PHOSPHORIC ACID MONO-[2-AMINO-3-(3H-IMIDAZOL-4-YL)-PROPYL]ESTER 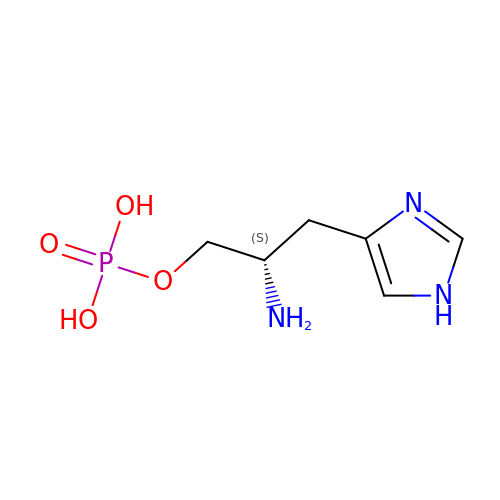| C6 H12 N3 O4 P | CWNDERHTHMWBSI-YFKPBYRVSA-N>DDGICKSSDCIKSAARLIQNMDATTEPCTDFFKYACGGWLKRNVIPETSSRYGNFDILRDELEVVLKDVLQEPKTEDIVAVQKAKALYRSCINESAIDSRGGEPLLKLLPDIYGWPVATENWEQKYGASWTAEKAIAQLNSKYGKKVLINLFVGTDDKNSVNHVIHIDQPRLGLPSRDYYECTGIYKEACTAYVDFMISVARLIRQEERLPIDENQLALEMNKVMELEKEIANATAKPEDRNDPMLLYNKMTLAQIQNNFSLEINGKPFSWLNFTNEIMSTVNISITNEEDVVVYAPEYLTKLKPILTKYSARDLQNLMSWRFIMDLVSSLSRTYKESRNAFRKALYGTTSETATWRRCANYVNGNMENAVGRLYVEAAFAGESKHVVEDLIAQIREVFIQTLDDLTWMDAETKKRAEEKALAIKERIGYPDDIVSNDNKLNNEYLELNYKEDEYFENIIQNLKFSQSKQLKKLREKVDKDEWISGAAVVNAFYSSGRNQIVFPAGILQPPFFSAQQSNSLNYGGIGMVIGHEITH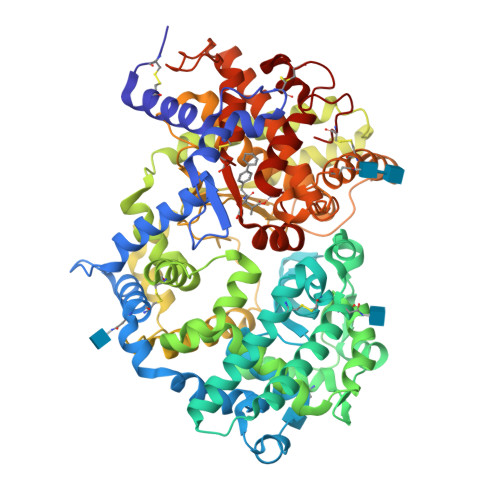GFDDNGRNFNKDGDLVDWWTQQSASNFKEQSQCMVYQYGNFSWDLAGGQHLNGINTLGENIADNGGLGQAYRAYQNYIKKNGEEKLLPGLDLNHKQLFFLNFAQVWCGTYRPEYAVNSIKTDVHSPGNFRIIGTLQNSAEFSEAFHCRKNSYMNPEKKCRVW[2x]>GSMHWNDLLNSNRRKPKNEKKESSQDTSKGRQQIERDYDRILFAAPTRRLADKTQVFPLDKNDSVRTRLTHSHEVANLSRGIGMRLAFELEDDVFKDVSEDICLKRDVPALLAAIGLVHDMGNPPFGAQGAKAMSEWFTKNLPEHSDNYKDKIYGDFRHFDGNSQTLRLVTKLQILNDTYGLNLTYATLASMIKYPRSSESDSSLWKKHGFFLSEKDVVQDIWNNTGLSEGVRHPFTYIMEACDDIAYSVLDAEDIIKKGFASFHDLIDFIQSNQFCKEDDVAKRVIENCKKIHADYAQQKLSPAELNDMSMQMFRVYAIAELVDAVVIAFKDNINEFLNDTCEIKDLISCSSGKNLCQALKKFDSSRGYQHRSVLKLELEGSNYIKGLMDMLWLGIKGRATGDTQYDTPFGRYVYGRISENYRRIFEQENNLPACYKEAQLLADAISGMTDSYLIALHDELRALHQYECRQR[8x]

pmcDeoxynucleoside triphosphohydrolase (dNTPase) enzymes are effector proteins in animal and bacterial cells that hydrolyze dNTP nucleotides and inhibit viral replication. We therefore named the dNTPase-NTase anti-phage defense system Clover and designated the dNTPase protein as Clover protein A (CloA) and the accessory NTase protein as Clover protein B (CloB). Likewise, CloA exhibits strict dGTP substrate specificity, with the activated enzyme only hydrolyzing dGTP and leaving other dNTPs including dTTP unaffected. Together these results demonstrate that CloA is a dGTPase effector that senses phage infection by specifically responding to elevated dTTP concentrations associated with viral replication. Clover defense encodes an accessory enzyme CloB that synthesizes an additional nucleotide signal p3diT that suppresses CloA activation and protects uninfected cells from aberrant nucleotide depletion. p3diT binds to CloA in an allosteric site adjacent to the dTTP binding pocket and raises the threshold of intracellular dNTP levels required to trigger full Clover immune activation.

To define the mechanism of nucleotide signaling in Clover anti-phage defense, we mutated the Salmonella CloA active site (H126A/E129A) to allow direct comparison of dGTP substrate interactions and determined cryo-EM structures of CloA in the suppressed CloA–dGTP–p3diT (2.6 Å) or activated CloA–dGTP–dTTP (2.6 Å) states. Remarkably, the CloA–dGTP–p3diT and CloA–dGTP–dTTP structures reveal that p3diT and dTTP each bind at the CloAAB interface in structurally distinct sites that remodel to accommodate the inhibiting or activating nucleotide signals. In the CloA–dGTP–p3diT suppressed state structure, p3diT is bound at the CloAAB interface in a pocket formed by helices α2A, α4B, α14B, and loop α1A–α2A that seals around the inhibitory nucleotide signal. Conserved residues from each CloA protomer form 10 hydrogen-bond interactions with p3diT that coordinate both the nucleotide signal 5′ triphosphate (CloA R34A, R38A, and N181A) and 3′–5′ phosphodiester linkage (R29A, R34A, and T25A). Specificity for p3diT binding is mediated by CloA residues that make base-specific contacts with the Watson-Crick edges of the first thymidine base T1 (Q311B) and second thymidine base T2 (D37A and N75B). CloA residues R314B and F41A further read-out the 3′ OH and deoxyribose sugar backbone of base T2. However, in the p3diT-bound suppressed state, the dGTP substrate is coordinated by comparatively minimal interactions between CloA residues that contact the guanosine nucleobase (Y246A and Q377A) and β- and γ-phosphates (Y193A, D243A, and K206A). In the p3diT bound suppressed state, interactions with the inhibitory nucleotide signal stabilize CloA loop α8A–α9A in an open conformation that is drawn away from the dTTP-binding site.Human ecto-5-nucleotidase (CD73) is involved in purinergic signalling, which influences a diverse range of biological processes. CD73 hydrolyses AMP and is the major control point for the levels of extracellular adenosine. CD73 is a non-covalent homodimer, which is attached via a glycosylphosphatidyl-inositol (GPI) anchor to the extracellular membrane. The N-terminal domain (residues 26–317) contains the metal-binding site, which can coordinate two zinc ions, whereas the C-terminal domain (residues 337–549) houses the substrate binding site.

We characterised the initial step of AMP hydrolysis, the binding mode of AMP to the open conformation of CD73 and compared that to other monophosphate substrates. The structure of CD73 in complex with AMP was determined to 1.69 Å resolution, and the AMP substrate is well defined by the electron density indicating full occupancy and no flexibility. The adenosine base is positioned by a π-stacking interaction with Phe417 and Phe500. There are no amino acid side chains within hydrogen bonding distance to the adenine ring, except for the interaction of N3 with the NH2-group of Asn390 at a rather long distance of 3.3 Å. The N1 of adenine interacts with the protein via two water molecules. The ribose group of AMP is positioned by hydrogen bonds with Asn390 and Asp506, whereas the phosphate group is coordinated by Arg354 and Arg395. An exception is Phe500, which exists in two conformations in the unliganded enzyme and the conformation with occupancy 0.36 disappears in the nucleotide-bound structure due to steric overlap with the adenine ring. Superposition of CD73open × AMP with CD73closed × AMPCP showed that the base and sugar moieties superimposed very well, confirming our structures to be a suitable means of studying the binding of alternative monophosphate substrates. In addition, concerning inhibitor development, it is evident, due to the optimal superposition of AMP and AMPCP between the open and closed form structures, that the open form is a suitable means for studying the binding of monophosphate nucleotides other than AMP to CD73. CD73 has a Km for AMP of 10.5 μM and a Vmax of 301.2 U/mg.

> MAHHHHHHVGTGSNDDDDKSPDPWELTILHTNDVHSRLEQTSEDSSKCVDASRCMGGVARLFTKVQQIRRAEPNVLLLDAGDQYQGTIWFTVYKGAEVAHFMNALRYDAMALGNHEFDNGVEGLIEPLLKEAKFPILSANISASGPLASQISGLYLPYKVLPVGDEVVGIVGYTSKETPFLSNPGTNLVFEDEITALQPEVDKLKTLNVNKIIALGHSGFEMDKLIAQKVRGVDVVVGGHSNTFLYTGNPPSKEVPAGKYPFIVTSDDGRKVPVVQAYAFGKYLGYLKIEFDERGNVISSHGNPILLDSSIPEDPSIKADINKWRIKLDDYSTQELGKTIVYLDGSSQSCRFRECNMGNLICDAMINNNLRHADEMFWNHVSMCILNGGGIRSPIDERNDGTITWENLAAVLPFGGTFDLVQLKGSTLKKAFEHSVHRYGQSTGEFLQVGGIHVVYDLSRKPGDRVVKLDVLCTSCRVPSYDPLKMDEVYKVILPNFLANGGDGFQMIKDELLRHDSGDQDINVVSTYISKMKVIYPAVEGRIKFS>GSHMDSTTIQQNKDTLSQIVVFPTGNYDKNEANAMVNRLANIDGKYLNALKQNNLKIKLLSGKLTDEKEYAYLKGVVPKGWEGTGKTWDDVPGLGGSTVALRIGFSNKGKGHDAINLELHATAHAIDHIVLNDISKSAQFKQIFAKEGRSLGNVNFLGVYPAEFFAESFAYYYLNQDTNSKLKSACPQTYSFLQNLAK[2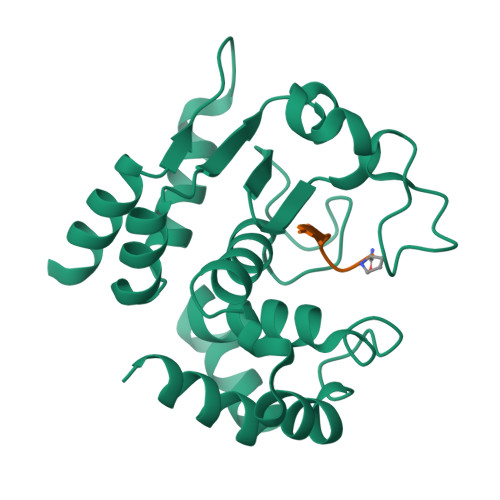x];>[2x]XEVNPPVP>TYFAPNSTGLRIQHGFETILIQPFGYDGFRVRAWPFRPPSGNEISFIYDPPIEGYEDTAHGMSYDTATTGTEPRTLRNGNIILRTTGWGGTTA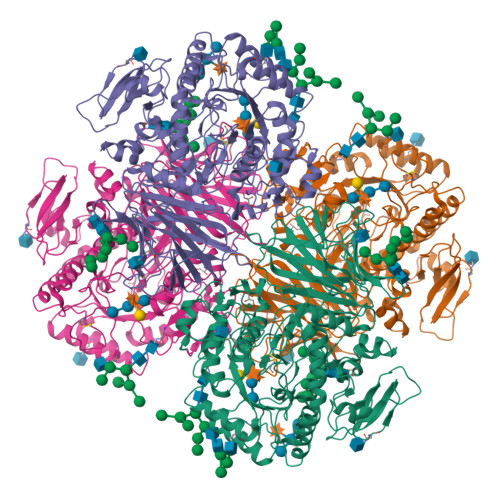GYRLSFYRVNDDGSETLLTNEYAPLKSLNPRYYYWPGPGAEFSAEFSFSATPDEQIYGTGTQQDHMINKKGSVIDMVNFNSYIPTPVFMSNKGYAFIWNMPAEGRMEFGTLRTRFTAASTTLVDYVIVAAQPGDYDTLQQRISALTGRAPAPPDFSLGYIQSKLRYENQTEVELLAQNFHDRNIPVSMIVIDYQSWAHQGDWALDPRLWPNVAQMSARVKNLTGAEMMASLWPSVADDSVNYAALQANGLLSATRDGPGTTDSWNGSYIRNYDSTNPSARKFLWSMLKKNYYDKGIKNFWIDQADGGALGEAYENNGQSTYIESIPFTLPNVNYAAGTQLSVGKLYPWAHQQAIEEGFRNATDTKEGSACDHVSLSRSGYIGSQRFCSMIWSGDTTSVWDTLAVQVASGLSAAATGWGWWTVDAGGFEVDSTVWWSGNIDTPEYRELYVRWLAWTTFLPFMRTHGSRTCYFQDAYTCANEPWSYGASNTPIIVSYIHLRYQLGAYLKSIFNQFHLTGRSIMRPLYMDFEKTDPKISQLVSSNSNYTTQQYMFGPRLLVSPVTLPNVTEWPVYLPQTGQNNTKPWTYWWTNETYAGGQVVKVPAPLQHIPVFHLGSREELLSGNVF[2x]>EDGKPVWAPHPTDGFQVGNIVDIGPDSLTIEPLNQKGKTFLALINQVFPAEEDSKKDVEDNCSLMYLNEATLLHNIKVRYSKDRIYTYVANILIAVNPYFDIPKIYSSETIKSYQGKSLGTMPPHVFAIADKAFRDMKVLKLSQSIIVSGESGAGKTENTKFVLRYLTESYGTGQDIDDRIVEANPLLEAFGNAKTVRNNNSSRFGKFVEIHFNEKSSVVGGFVSHYLLEKSRICVQGKEERNYHIFYRLCAGASEDIRERLHLSSPDNFRYLNRGCTRYFANKETDKQILQNRKSPEYLKAGSLKDPLLDDHGDFIRMCTAMKKIGLDDEEKLDLFRVVAGVLHLGNIDFEEAGSTSGGCNLKNKSTQALEYCAELLGLDQDDLRVSLTTRVMLTTAGGAKGTVIKVPLKVEQANNARDALAKTVYSHLFDHVVNRVNQCFPFETSSYFIGVLDIAGFEYFEHNSFEQFCINYCNEKLQQFFNERILKEEQELYQKEGLGVNEVHYVDNQDCIDLIEARLVGILDILDEENRLPQPSDQHFTSAVHQKHKDHFRLSIPRKSKLAIHRNIRDDEGFIIRHFAGAVCYETTQFVEKNNDALHMSLESLICESRDKFIRELFESSTNNNKDTKQKAGKLSFISVGNKFKTQLNL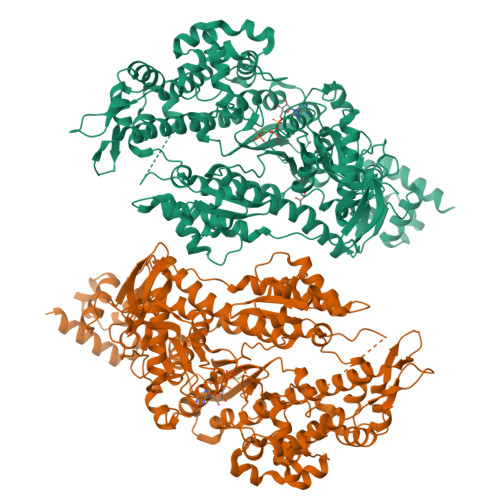LLDKLRSTGASFIRCIKPNLKMTSHHFEGAQILSQLQCSGMVSVLDLMQGGFPSRASFHELYNMYKKYMPDKLARLDPRLFCKALFKALGLNEIDYKFGLTKVFFRPGKFAEFDQIMKSDPDHLAELVKRVNHWLI[2x]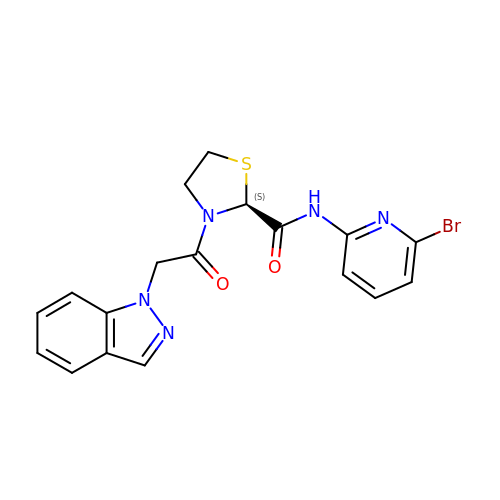(2S)-N-(6-bromopyridin-2-yl)-3-[(1H-indazol-1-yl)acetyl]-1,3-thiazolidine-2-carboxamide | C18 H16 Br N5 O2 S | JSZBVXMPHMCOIC-SFHVURJKSA-N>[3x]PKHGKRYRAL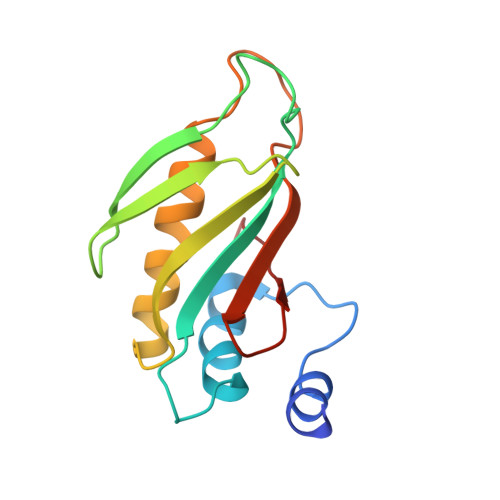LEKVDPNKIYTIDEAAHLVKELATAKFDETVEVHAKLGIDPRRSDQNVRGTVSLPHGGRIEFRNDKTGAIHAPVGKASFPPEKLADNIRAFIRALEAHKPEGAKGTFLRSVYVTTTMGPSVRINPHS Bromodomains (BRDs) are protein interaction modules that specifically recognize ε-N-lysine acetylation motifs, a key event in the reading process of epigenetic marks. The 61 BRDs in the human genome cluster into eight families based on structure/sequence similarity. Despite large sequence variations, all BRD modules share a conserved fold that comprises a left-handed bundle of four α helices (αZ, αA, αB, αC), linked by loop regions of variable length (ZA and BC loops), which line the Kac binding site and determine binding specificity. The four helices form a deep cavity that is extended by the two loop regions (ZA and BC loops), creating a largely hydrophobic Kac binding pocket.

Cocrystal structures with peptides have demonstrated that Kac is recognized by a central deep hydrophobic cavity, where it is anchored by a hydrogen bond to an asparagine residue present in most BRDs (Owen et al., 2000). An asparagine residue that anchors Kac by formation of a critical hydrogen bond initiates the BC loop. Indeed, ITC experiments showed that the binding affinity of many BRDs was significantly increased for multiply modified peptides. For example, the KD of CREBBP decreased from 733 μM for H3K14ac to 131 μM for H3pS10K14acK18ac suggesting that many BRDs recognize a pattern of modifications rather than a single Kac mark.

>[2x]SMRKKIFKPEELRQALMPTLEALYRQDPESLPFRQPVDPQLLGIPDYFDIVKNPMDLSTIKRKLDTGQYQEPWQYVDDVWLMFNNAWLYNRKTSRVYKFCSKLAEVFEQEIDPVMQSLG> TEFKAGSAKKGATLFKTRCLQCHTFDQGGAN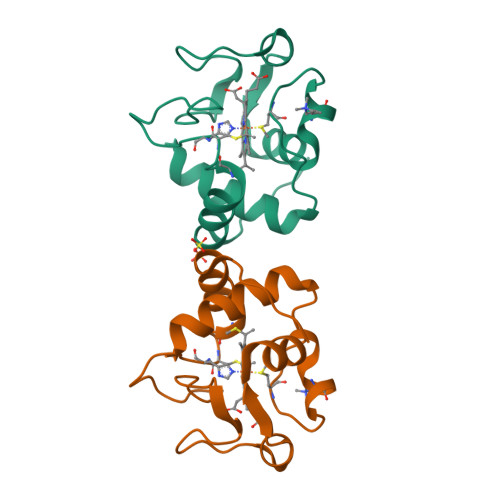KVGPNLHGIFGRHSGQAEGYSYTDANIKKNVLWDENNMSEYLTNPKKYIPGTKMAFGGLKKEKDRNDLITYLKKACE> MITMKCRKCGKPSIYHQKHSGNNYCKECFIKETKRKVRKTLGRDVLKNNIKVAMGLSGGKDSLVMAYLL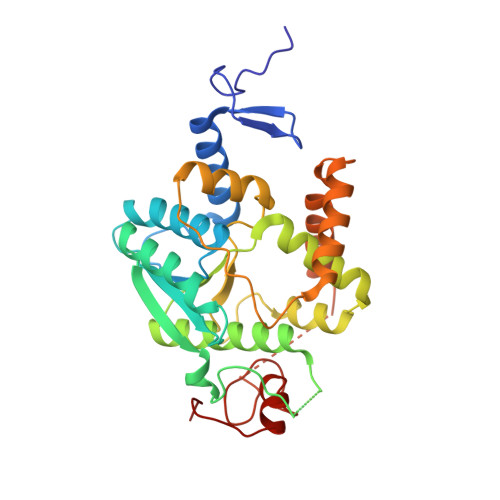NEYYKQIPNSNLIAIMVNEGIEGYRTDGIDAAVKFCEEYGIEYKIVHFKDYLGTNLDEIVKIAKEKNLTMNPCSFCGVIRRKILNRVSIEEKCDFLAIGHNLDDVAQAVMMNYIEGDVKKLAFLGKSLKHPKFVKRIKPLEKIPEDEVLLLAEMLELKYHKSPCPYSCLSFRSEVSDITDNLEKNHPGSKYSIVRGYERLLEHIELPGYTGECKICGGLSATEVCKVCSYGKNLGILEKSKF N-(3-MERCAPTOPROPANOYL)-D-ALANINE 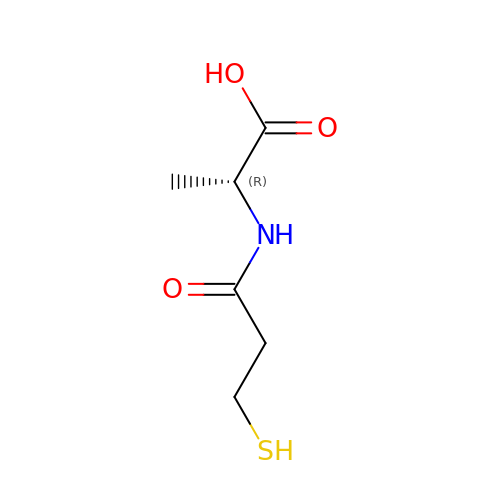| C6 H11 N O3 S | JIAFOCJABIEPNM-SCSAIBSYSA-N> MVRGIRGAITVEEDTPEAIHQATRELLLKMLEANGIQSYEELAAVIFTVTEDLTSAFPAEAARQIGMHRVPLLSARE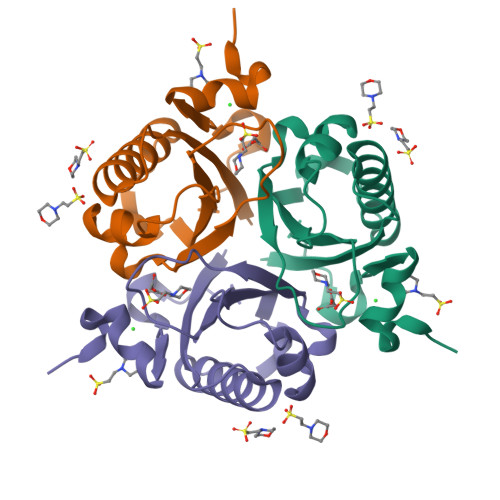VPVPGSLPRVIRVLALWNTDTPQDRVRHVYLREAVRLRPDLESAQ> GPMAIGLPSINISFKELATTVKERSARGIIAMVLKDAKALGLNEIHEKEDIPVDLSAENKEYINLALMGNVNTPNKLLVYVIEGEADIQTALDFLETKEFNYLCMPKAVEADKTAIKNWIIKLRDIDKVKVKAVLGKVVGNHEGIINFTTEDVLVGEKKYSVDEFTSRVAGLIAGTPLSQSVTYTKLSDVVDIPKMTKVDAESKVNKGELILIKEAGAIRIARGVNSLTELTAEKGEMFQKIKIVDTLDIIHSDIRKVIIDDYIGKVTNSYDNKCLLIVAIKSYLEELEKSALIESDSTVEIDFEAQKSYLKSKGVDLSYMTLQEIKEANTGSKVFLKAKIKVLDAMEDIDLSIEI

A rather recently identified group of PTLBs are the R-type “diffocins” from Clostridium difficile, which constitute the only Gram-positive R-type PTLBs known to date. All R-type PTLBs consist of an inner needle-like rigid tube surrounded by a contractile sheath. Binding triggers extensive conformational changes in the baseplate, accompanied by contraction of the sheath, which, due to extensive interactions, drives the rigid inner tube into the cell envelope. Here, we have determined the crystal structures and SAXS envelopes of the R-type diffocin tube and sheath protein CD1364 and CD1363 in their pre-assembled monomeric state.

The R-type diffocin sheath protein CD1363 crystallized in space group C121 with one molecule in the asymmetric unit. Therefore, SAD data were collected from a crystal obtained from SeMet-labeled CD1363 protein. Because crystals of the labeled protein diffracted to higher resolution, the structure was refined against these data and the subsequent discussion refers to SeMet-labeled CD1363. In the crystal form discussed here, CD1363 is monomeric and comprises two domains. The domain arrangement is best described as a “Russian doll” system in which domain II (residues G26–S225; domain numbering according to Leiman and Shneider, 2012) is an insertion into domain I (residues G4–R25 and residues L226–I354). At the N-terminus, residues P6–A25 form a long α-helix that closely interacts with α-helices α9 and α10, which flank the central antiparallel three-stranded β-sheet. The larger domain II is composed of a central six-stranded β-sheet and five smaller β-strands flanked by four and two α-helices, respectively. Similar mesh-like organizations have been found in several T6SSs, indicating that these interactions are likewise conserved in assembled R-type PTLBs. Interestingly, the C-terminus in monomeric CD1363 also forms a β-strand (β14) that hydrophobically interacts with residues of α9 and α10 as well as with the same residues from the neighboring β-strand (β13 in CD1363) as observed in the pyocin particle, albeit within the same chain (Figure 3A magnified insert and Figure 3B).>[3x]MGAVAVDLGNRKLEISSGKLARFADGSAVVQSGDTAVMVTAVSKTKPSPSQFMPLVVDYRQKAAAAGRIPTNYLRREVGTSDKEILTSRIIDRSIRPLFPAGYFYDTQVLCNLLAVDGVNEPDVLAINGASVALSLSDIPWNGPVGAVRIGIIDGEYVVNPTRKEMSSSTLNLVVAGAPKSQIVMLEASAENILQQDFCHAIKVGVKYTQQIIQGIQQLVKETGVTKRTPQKLFTPSPEIVKYTHKLAMERLYAVFTDYEHDKVSRDEA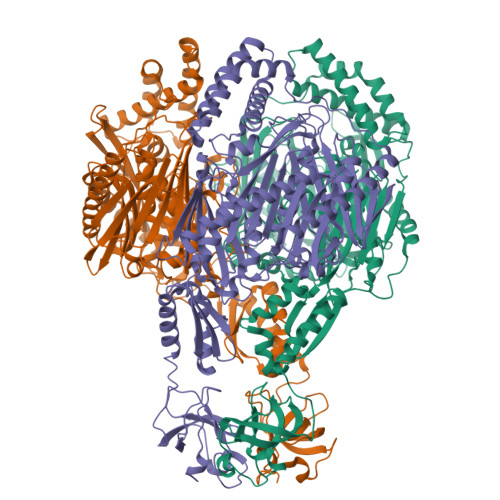VNKIRLDTEEQLKEKFPEADPYEIIESFNVVAKEVFRSIVLNEYKRCDGRDLTSLRNVSCEVDMFKTLHGSALFQRGQTQVLCTVTFDSLESGIKSDQVITAINGIKDKNFMLHYEFPPYATNEIGKVTGLNRRELGHGALAEKALYPVIPRDFPFTIRVTSEVLESNGSSSMASACGGSLALMDSGVPISSAVAGVAIGLVTKTDPEKGEIEDYRLLTDILGIEDYNGDMDFKIAGTNKGITALQADIKLPGIPIKIVMEAIQQASVAKKEILQIMNKTISKPRASRKENGPVVETVQVPLSKRAKFVGPGGYNLKKLQAETGVTISQVDEETFSVFAPTPSAMHEARDFITEICKDDQEQQLEFGAVYTATITEIRDTGVMVKLYPNMTAVLLHNTQLDQRKIKHPTALGLEVGQEIQVKYFGRDPADGRMRLSRKVLQSPATTVVRTLNDRSSIVMGEPISQSSSNSQAAALEHHHHHH>SNAMLRRLFKKKYVCVRQYDLTDCGAACLSSIAQYYGLKMSLAKIREMTGTDTQGTNAYGLIHAAKQLGFSAKGVKASKEDLLKDFRLPAIANVIVDNRLAHFVVIYSIKNRIITVADPGKGIVRYSMDDFCSIWTGGLVLLEPGEAFQKGDYTQNMMVKFAGFLKPLKKTVLCIFLASLLYTALGIAGSFYIKFLFDDLIKFEKLNDLHIISAGFAVIFLLQIFLNYYRSILVTKLGMSIDKSIMMEYYSHVLKLPMNFFNSRKVGEIISRFMDASKIRQAISGATLTIMIDTIMAVIGGILLYIQNSSLFFISFIIILLYGIIVTVFNKPIQNANRQIMEDNAKLTSALVESVKGIETIKSFGAEEQTEKSTRDKIETVMKSSFKEGMLYINLSSLTGIVAGLGGIVILWAGAYNVIKGNMSGGQLLAFNALLAYFLTPVKNLIDLQPLIQTAVVASNRLGEILELATEKELREDSDDFVISLKGDIEFRNVDFRYGLRKPVLKNINLTIPKGKTVAIVGESGSGKTTLAKLLMNFYSPEKGDILINGHSIKNISLELIRKKIAFVSQDVFIFSGTVKENLCLGNENVDMDEIIKAAKMANAHDFIEKLPLKYDTFLNESGANLSEGQKQRLAIARALLKKPDILILDEATSNLDSITENHIKDAIYGLEDDVTVIIIAHRLSTIVNCDKIYLLKDGEIVESGSHTELIALKGCYFKMWKQTENTLAS[2x];>[2x]SNAMSEAKKLNIGRELTDEELMEMTGGSTFSIQCQKDYTYKPSLPVVKYGVVIDEPEVV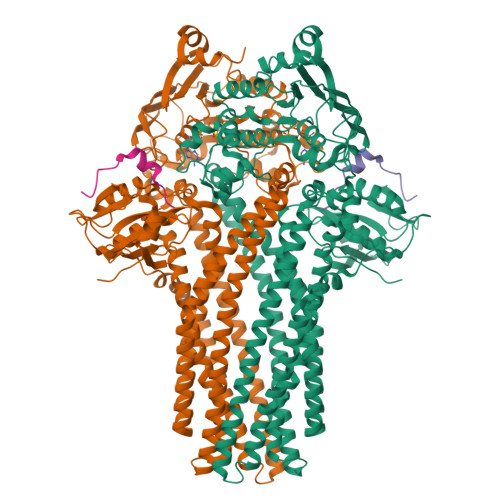IKYGVGPIVGIKYGVEPIGPIQPMYGIKPVETLK> MTKKVGVGQAHSKIILIGEHAVVYGYPAISLPLLEVEVTCKVVPAESPWRLYEEDTLSMAVYASLEYLNITEACIRCEIDSAIPEKRGMGSSAAISIAAIRAVFDYYQADLPHDVLEILVNRAEMIAHMNPSGLDAKTCLSDQPIRFIKNVGFTELEMDLSAYLVIADTGVYGHTREAIQVVQNKGKDALPFLHALGELTQQAEIAISQKDAEGLGQILSQAHLHLKEIGVSS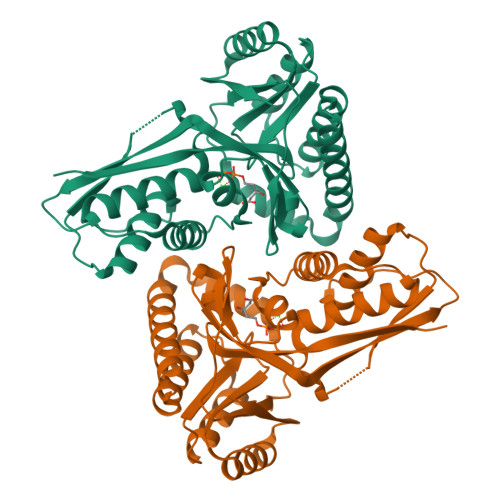LEADSLVETALSHGALGAKMSGGGLGGCIIALVTNLTHAQELAERLEEKGAVQTWIESL> GSMSAHNWDNELSGIQNTSVSLAADYVYMRLATEGFVFGIRSSVRAPIRLCDAMFLMCDLFERKFHDRYIAPLKNACLGISAKDMDM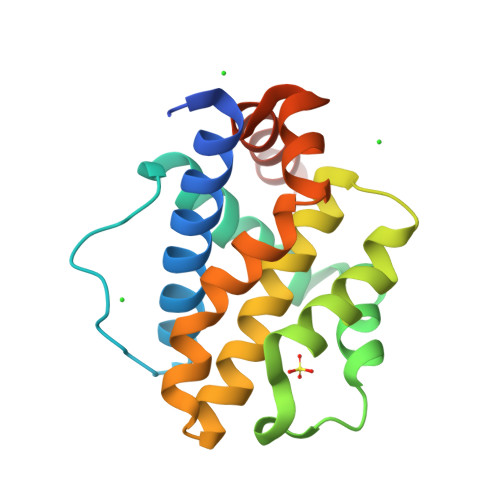RMFFSALDSVFSSGISWSRIVAMYAFAGSVALACARQGRRQTVIAIPEWIMLYMRRAIAPWIHANGGWDSFIKFSQDVLNGNHEEDG2-BROMO-2-PROPENE-1-OL | C3 H5 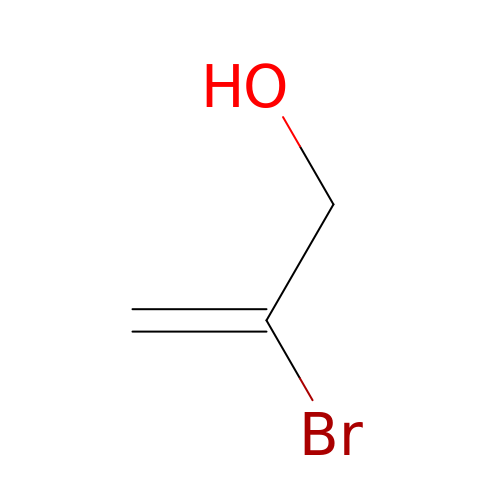Br O | MDFFZNIQPLKQSG-UHFFFAOYSA-N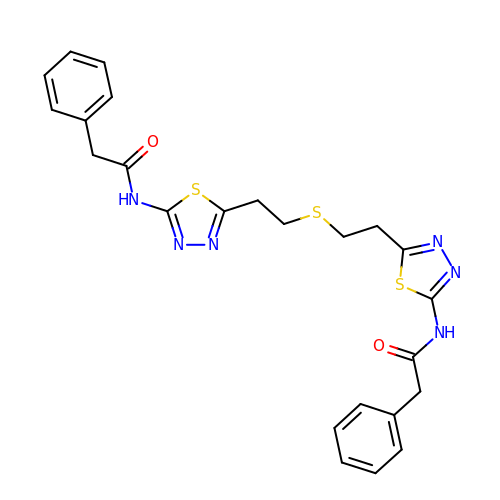N,N'-[sulfanediylbis(ethane-2,1-diyl-1,3,4-thiadiazole-5,2-diyl)]bis(2-phenylacetamide) | C24 H24 N6 O2 S3 | MDJIPXYRSZHCFS-UHFFFAOYSA-N>TKHKERVMYYGKGDVFAYRTYLKPLTGVRTIPESPFSGRDHILFGVNVKISVGGTKLLTSFTKGDNSLVVATDSMKNFIQKHLASYTGTTIEGFLEYVATSFLKKYSHIEKISLIGEEIPFETTFAVKNGNRAASELVFKKSRNEYATAYLNMVRNEDNTLNITEQQSGLAGLQLIKVSGNSFVGFIRDEYTTLPEDSNRPLFVYLNIKWKYKNTEDSFGTNPENYVAAEQIRDIATSVFHETETLSIQHLIYLIGRRILERFPQLQEVYFESQNHTWDKIVEEIGESEGK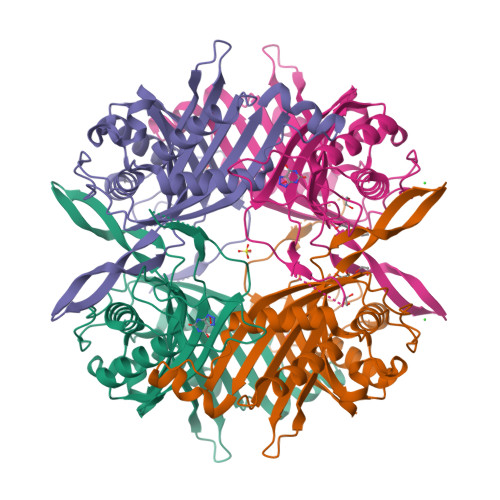VYTEPRPPYGFQCFTVTQEDLPHENILMFSDE[2x]>MEKRIKGSCTSILVGKKASIDGSTLISRNDDGHEALDPQRFVVVNPEDQPRDYTSVISKVNVKLPDDPQRYTSIPNSILTNGIWPAAGINSSNVAMSATETITTNSRVQGLDPFVENGLGEEDLVTVVLPYVKSAREGVKRLGSLLEEYGTYEPNGISFADNEEVWWLETIGGHHWAAVRIPDDAYVVAPNRMNIDQFDFDSDDTLCSSDLKDLIDNNNLNPDFENYNLRHIFGSASIKDTVYNNPRTWYGQKFFSPDDTADDPMEQDLPFICHANRKISVEDVKFVLSSHFENTKYDVY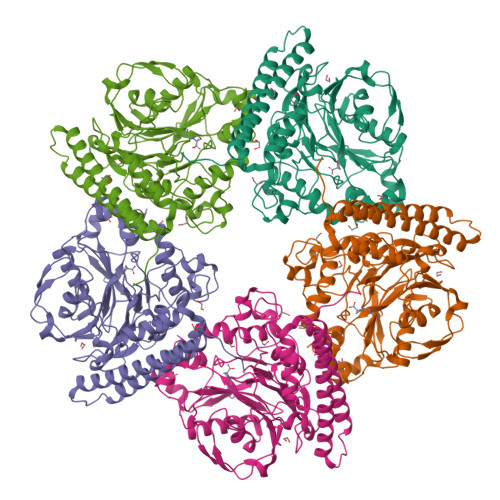GSGSQSDKTLFRPIGINRNHNVHILQIRNNVPTEIAGIHWLAYGANTFNTVVPFYANVNDTPVQYKNATGKFDLNNMYWLSCTTALLGDTDYDFYVDMRNDYELDAMSAYRKIQNDTDADISGQKDIEKYLENANKKLADVAFEKQNKLLGDMVTTGSNNMKLRYNLND[5x]(3S,5R)-N-(2,2-diphenylethyl)-5-{[(4-methylphenyl)sulfonyl]amino}piperidine-3-carboxamide | C27 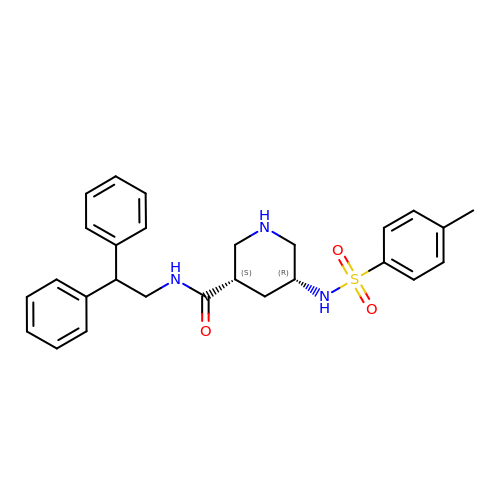H31 N3 O3 S | TUYPQRDSHLXMFM-BJKOFHAPSA-N5-(6-AMINO-9H-PURIN-9-YL)-4-HYDROXYTETRAHYDROFURAN-3-YL DIHYDROGEN PHOSPHATE 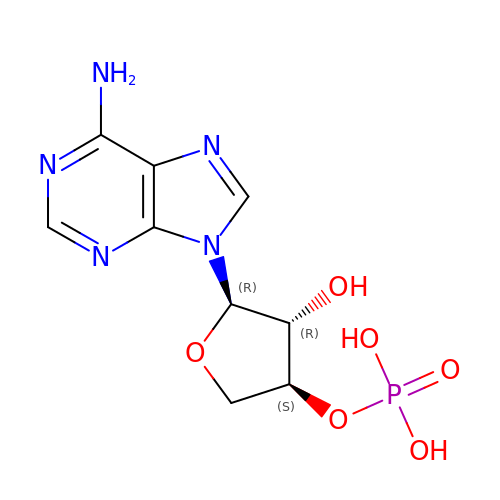| C9 H12 N5 O6 P | IJEJRDCFMFEDGL-AFEQZKEHSA-N>MSISASEARQRLFPLIEQVNTDHQPVRITSRAGDAVLMSADDYDAWQETVYLLRSPENARRLMEAVARDKAGHSAFTKSVDELREMAGGEEMQAGPAL[8x];>[8x]HHHHHHDDDDKVRSVNFDPDAWEDFLFWLAADRKTARRITRLIGEIQRDPFSGIGKPEPLQG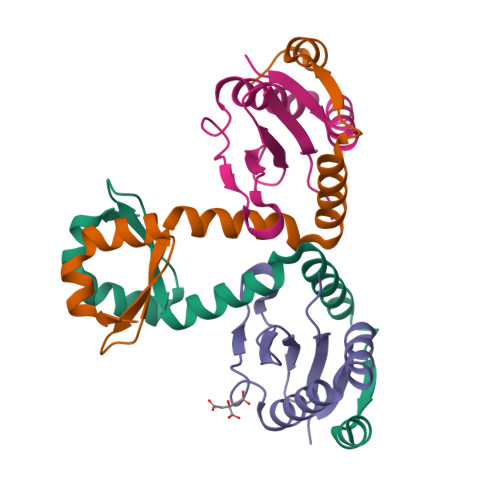ELSGYWSRRIDDEHRLVYRAGDDEVTMLKARYHY> ATYAMGSMRVLLALHDRAPQLKISDDRLTVVGEKGYSMVRASHGVRKGAWYFEITVDEMPPDTAARLGWSQPLGNLQAPLGYDKFSYSWRSKKGTKFHQSIGKHYSSGYGQGDVLGFYINLPEDTISGRGSEIIFYKNGVNQG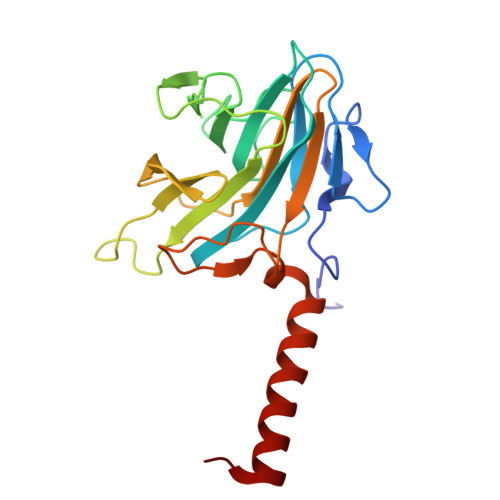VAYKDIFEGVYFPAISLYKSCTVSINFGPCFKYPPKDLTYRPMSDMGWGAVVEHTLADVLYHVETEVDGRR> DVPVNLYRPNAPFIGKVISNEPLVKEGGIGIVQHIKFDLTGGNLKYIEGQSIGIIPPGVDKNGKPEKLRLYSIASTRHGDDVD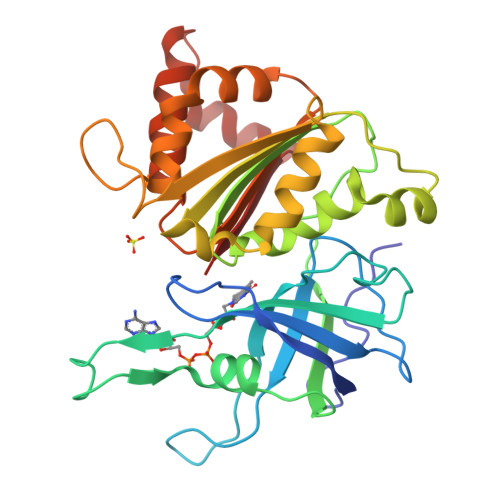DKTISLCVRQLEYKHPESGETVYGVCSTYLTHIEPGSEVKITGPVGKEMLLPDDPEANVIMLAGGTGIAPMRTYLWRMFKDAERAANPEYQFKGFSWLVFGVPTTPNILYKEELEEIQQKYPDNFRLTYAISREQKNPQGGRMYIQDRVAEHADQLWQLIKNQKTHTYICGLRGMEEGIDAALSAAAAKEGVTWSDYQKDLKKAGRWHVETY(1S,2S)-2-(3-fluorobenzyl)-N-{2-[2-(1H-imidazol-1-yl)pyrimidin-4-yl]ethyl}cyclopropanamine 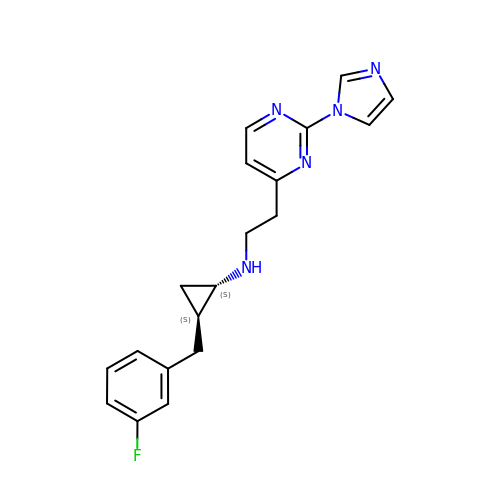| C19 H20 F N5 | CYEVFFVOLRMDHH-YJBOKZPZSA-N>GSHNDKDLSTWQTFRRLWPTIAPFKAGLIVAGVALILNAASDTFMLSLLKPLLDDGFGKTDRSVLVWMPLVVIGLMILRGITSYVSSYCISWVSGKVVMTMRRRLFGHMMGMPVSFFDKQSTGTLLSRITYDSEQVASSSSGALITVVREGASIIGLFIMMFYYSWQLSIILIVLAPIVSIAIRVV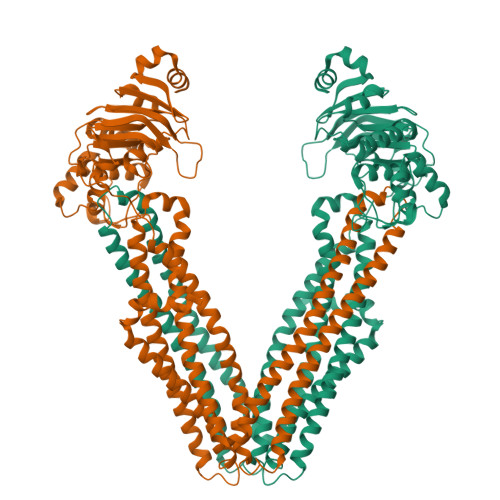SKRFRNISKNMQNTMGQVTTSAEQMLKGHKEVLIFGGQEVETKRFDKVSNRMRLQGMKMVSASSISDPIIQLIASLALAFVLYAASFPSVMDSLTAGTITVVFSSMIALMRPLKSLTNVNAQFQRGMAACQTLFTILDSEQEKDEGKRVIERATGDVEFRNVTFTYPGRDVPALRNINLKIPAGKTVALVGRSGSGKSTIASLITRFYDIDEGEILMDGHDLREYTLASLRNQVALVSQNVHLFNDTVANNIAYARTEQYSREQIEEAARMAYAMDFINKMDNGLDTVIGENGVLLSGGQRQRIAIARALLRDSPILILDEATSALDTESERAIQAALDELQKNRTSLVIAHRLSTIEKADEIVVVEDGVIVERGTHNDLLEHRGVYAQLHKMQFGQ[2x]>[18x]MDPFLVLLHSVSSSLSSSELTELKFLCLGRVGKRKLER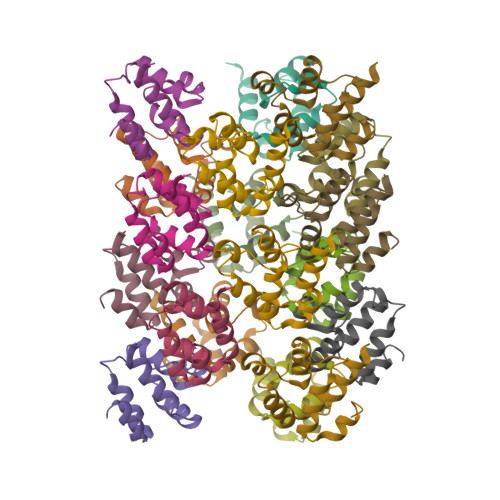VQSGLDLFSMLLEQNDLEPGHTELLRELLASLRRHDLLRRVDDFEAGAAAGAA>[2x]MHHHHHHHHAMSNSKFNVRLLTEIAFMAALAFIISLIPNTVYGWIIVEIACIPILLLSLRRGLTAGLVGGL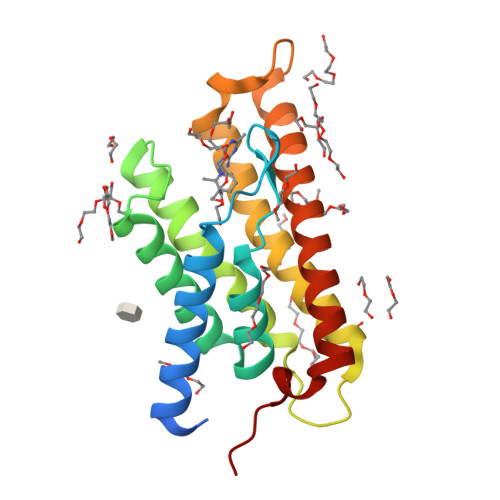IWGILSMITGHAYILSLSQAFLEYLVAPVSLGIAGLFRQKTAPLKLAPVLLGTFVAVLLKYFFHFIAGIIFWSQYAWKGWGAVAYSLAVNGISGILTAIAAFVILIIFVKKFPKLFIHSNY>[3x]MGQVEVFNGQDTRDGVNILIMGTDGRIGQNSVETRTDSIMVLNVGGSDKKMKLVSFMRDNLVYIDGYSQVINGRKQTDNKLNVAYELGEQEGQKGAEMVRQVLKDNFDLDIK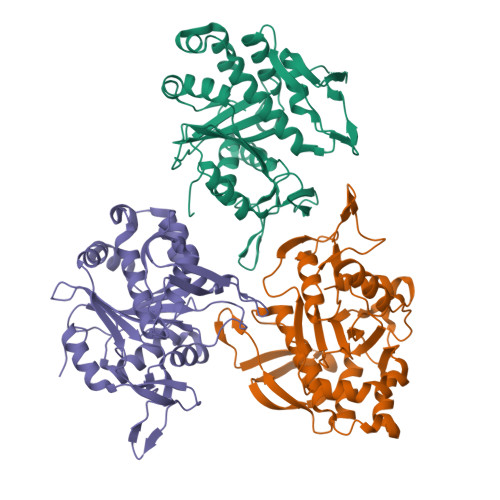YYALVDFQAFATAIDTLFPDGVTIDAQFSTLNGRPLTEATVGDDLYATETESPTQTIKVGKQQMNGSTLLNYARFRDDDEADYGRTKRQQQVLTAILEQIKDPTKLFTGSEALGKVFAMTSTNVPYTFLLTNGLSVLDGAKNGIEKLTIPELGDWVDAYDVYGGLGLLVDQNKYQTKLAQMGLRAAALEHHHHHH> ARGSHMEEMIRSLQQRPEPTPEEWDLIHIATEAHRSTNAQGSHWKQRRKFLPDDIGQSPIVSMPDGDKVDLEAFSEFTKIITPAITRVVDFAKKLPMFSELPCEDQIILLKGCCMEIMSLRAAVRYDPESDTLTLSGEMAVKREQLKNGGLGVVSDAIFELGKSLSAFNLDDTEVALLQAVLLMSTDRSGLLCVDKIEKSQEAYLLAFEHYVNHRKHNIPHFWPKLLMKVTDLRMIGACHASRFLHCKVECPTELFPPLFL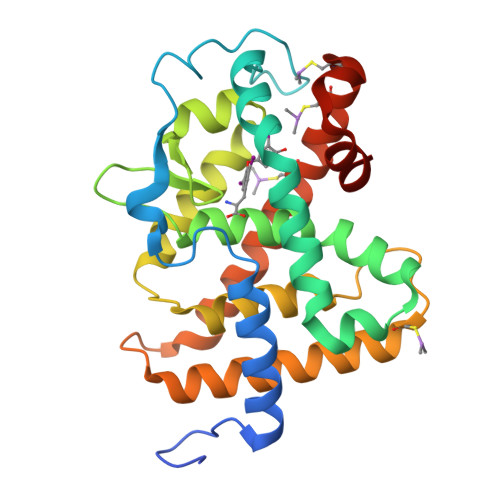EVFEDQEV> MGSSHHHHHHSQDPMVLLHKSTHIFPTDFASVSRAFFNRYPNPYSPHVLSIDTISRNVDQEGNLRTTRLLKKSGKLPTWVKP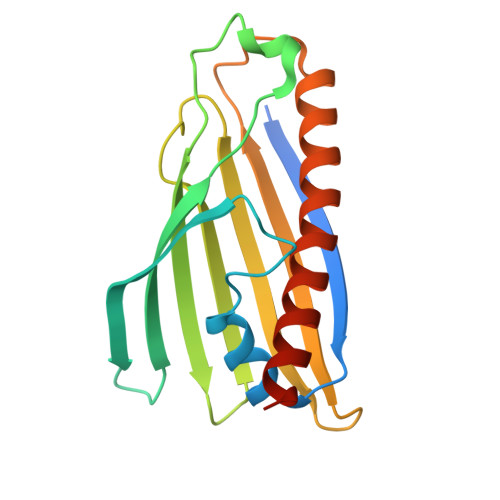FLRGITETWIIEVSVVNPANSTMKTYTRNLDHTGIMKVEEYTTYQFDSATSSTIADSRVKFSSGFNMGIKSKVEDWSRTKFDENVKKSRMGMAFVIQKLEEARNPQF>MAETPNSDMSGATGGRSKRPKSNQDWWPSKLNLEILDQNARDVGPVEDDFDYAEEFQKLDLEAVKSDLEELMTSSQDWWPADYGHYGPLFIRMAWHSAGTYRTADGRGGAAGGRQRFAPINSWPDNANLDKARRLLLPIKQKYGQKISWADLMILAGNVAIESMGFKTFGYAGGREDAFEEDKAVNWGPEDEFETQERFDEPGEIQEGLGASVMGLIYVNPEGPDGNPDPEASAKNIRQTFDRMAMNDKETAALIAGGHTFGKVHGADDPEENLGPEPEAAPIEQQGLGWQNKNGNSKGGEMITAGIEGPWTQSPTEWDMGYINNLLDYEWEPEKGPGGAWQWAPKSEELKNSVPDAHDPDEKQTPMMLTTDIALKRDPDYREVMETFQENPMEFGMNFAKAWYKLTHRDMGPPERFLGPEVPDEEMIWQDPLPDADYDLIGDEEIAELKEEILDSDLSVSQLVKTAWASASTYRDSDKRGGANGARLRLEPQKNWEVNEPEQLETVLGTLENIQTEFNDSRSDGTQVSLADLIVLGGNAAVEQAAANAGYDVEIPFEPGRVDAGPEHTDAP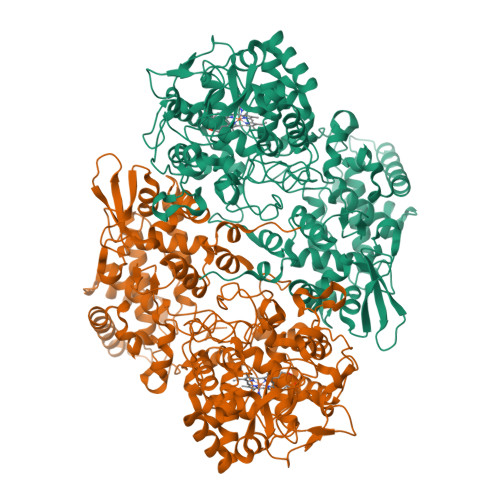SFDALKPKVDGVRNYIQDDITRPAEEVLVDNADLLNLTASELTALIGGMRSIGANYQDTDLGVFTDEPETLTNDFFVNLLDMGTEWEPAADSEHRYKGLDRDTGEVKWEATRIDLIFGSNDRLRAISEVYGSADAEKKLVHDFVDTWSKVMKLDRFDLEHHHHHH[2x]>[7x]XGEIAQGIKEIAKGIKEIAWGIKEIAKGIKGX

Expanding this pattern to hpphhph can produce larger α-helical barrels. Here, we show that pentameric to nonameric barrels are accessed by varying the residue at one of the h sites. In peptides with four L/I–K–E–I–A–x–Z repeats, decreasing the size of Z from threonine to serine to alanine to glycine gives progressively larger oligomers. X-ray crystal structures of the resulting α-helical barrels rationalize this: side chains at Z point directly into the helical interfaces, and smaller residues allow closer helix contacts and larger assemblies.

Conversely, both Gly variants scored more favourably as larger oligomeric states: the a = d = Ile variant as an octamer; and a = Leu, d = Ile as a nonamer. The Gly@g variant with a = d = Ile unfolded at 38 °C and did not fully refold on cooling. Indeed, peptide sequences with a = d = Ile are more unstable than their a = Leu, d = Ile counterparts. Thus, β-branched Ile at both a and d maintains the open assembly even with Gly residues at g. Although a larger oligomer was predicted in silico, the calculated internal energies for Gly@g were similar for the different oligomers (Fig. S1†). The hexameric and heptameric assemblies of CC-Type2-(GgIaId)4 imply that, whilst Gly@g is necessary to access larger states, it is not the only factor that dictates oligomer state of the helical assembly.>[2x]GSQIPASEQETLVRPKPLLLKLLKSVG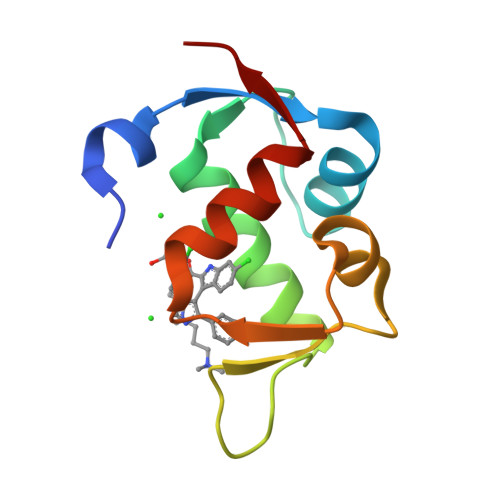AQKDTYTMKEVLFYLGQYIMTKRLYDEKQQHIVYCSNDLLGDLFGVPSFSVKEHRKIYTMIYRNLVVVN DIETHYL HYDROGEN PHOSPHATE | C4 H11 O4 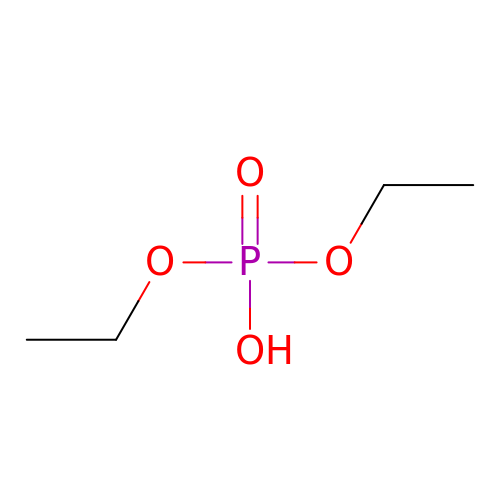P | UCQFCFPECQILOL-UHFFFAOYSA-N> MECISVKGRIYSILKQIGSGGSSKVFQVLNEKKQIYAIKYVNLEEADNQTLDSYRNEIAYLNKLQQHSDKIIRLYDYEITDQYIYMVMECGNIDLNSWLKKKKSIDPWERKSYWKNMLEAVHTIHQHGIVHSDLKPANFLIVDGMLKLIDFGIANQMQPDTTSVVKDSQVGTVNYMPPEAIKDMSSSRENGKSKSKISPKSDVWSLGCILYYMTYGKTPFQQIINQISKLHAIIDPNHEIEFPD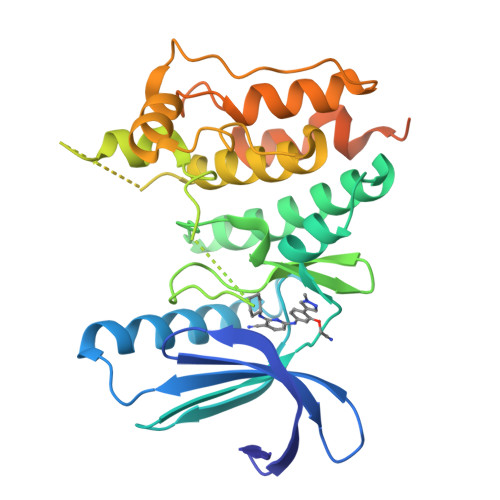IPEKDLQDVLKCCLKRDPKQRISIPELLAHPYVQIQTHPVNQMAKGTTEEMKYVLGQLVGLNLVPRGSAAGHHHHHH>STAGKVIKCKAAVLWELKKPFSIEEVEVAPPKAHEVRIKMVAVGICGTDDHVVSGTMVTPLPVILGHEAAGIVESVGEGVTTVKPGDKVIPLAIPQCGKCRICKNPESNYCLKNDVSNPQGTLQDGTSRFTCRRKPIHHFLGISTFSQYTVVDENAVAKIDAASPLEKVCLIGCGFSTGYGSAVNVAKVTPGSTCAVFGLGGVGLSAIMGCKAAGAARIIAVDINK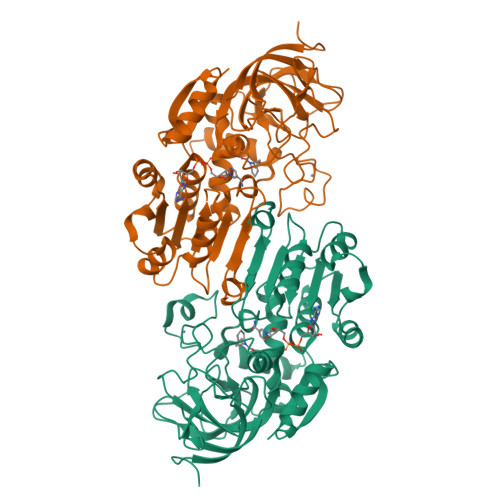DKFAKAKELGATECINPQDYKKPIQEVLKEMTDGGVDFSFEVIGRLDTMMASLLCCHEACGTSVIVGVPPDSQNLSMNPMLLLTGRTWKGAILGGFKSKECVPKLVADFMAKKFSLDALITHVLPFEKINEGFDLLHSGKSIRTILMF[2x]>CCGGGAC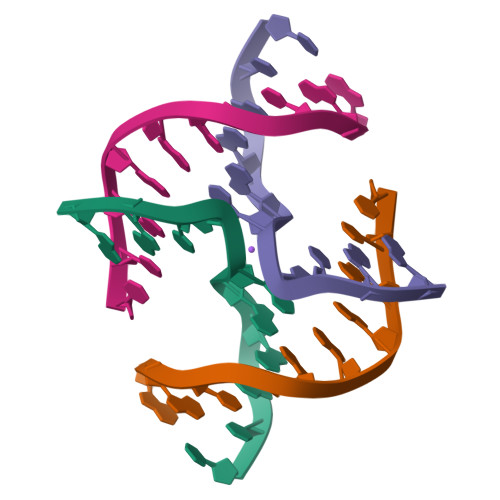CGG[2x]4'-HYDROXYCINNAMIC ACID | C9 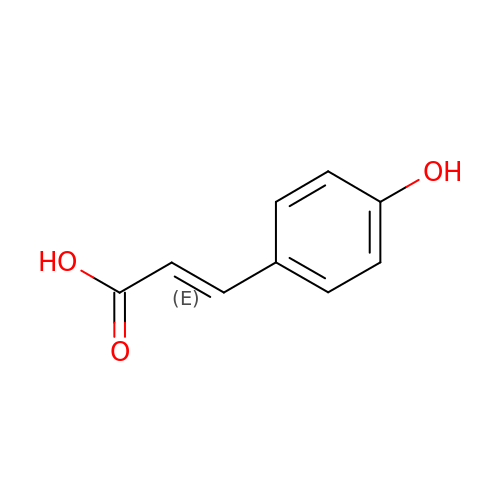H8 O3 | NGSWKAQJJWESNS-ZZXKWVIFSA-N> PLTEQEIDELCDEWVPEPLIPPITEDMKHEPPVLESAAGPHTTVNGKDVVNFASANYLGLIGHEKLLESCTSALEKYGVGSCGPRGFYGTIDVHLDCETRISKFLGTPDSILYSYGLSTMFSTIPCFCKKGDVIVADEGVHWGIQNGLQLSRSTIVYFKHNDMESLRITLEKIMTKYKRSKNLRRYIVAEAVYQNSGQIAPLDEIVKLKEKYRFRVILDESNSFGVLGRSGRGLAEHHSVPIEKIDVVTAAMGHALATEGGFCTGNARIIDYQRLSSSGYVFSASLPPYLASAAITAIDVIDQNPDMLVKLKQNVALLWKGLSDIKGMSLTSNRESPIVFLKLEKSSGSAKDDLLLLEKMADRALKEDSLLVVSSKRSFLDKCRLPVGIKLYVSAGHSESDLLKASESLKRLASELLLKS;> MYLTAVSTYFSYGLLFAFGQLRDFFRRFIDWWFTSNLQGYAPICLGHEDFYIRRLYHRIQDCFERPISSAPDAWFDVVERYSNDNNKTLKRTTKTSRCLNLGSYNYLGFGSFDEYCTPRVIESLKKFSASTCSSRVDAGTTSVHAELEECVTRFVGKPAAVVFGMGYATNSAIIPVLIGKGGLIISDSLNHSSIVNGARGSGATIRVFQHNTPSHLERVLREQIAEGQPRTHRPWKKIIVVVEGIYSMEGEICHLPEVVAICKKYKAYVYLDEAHSIGAIGKTGKGICELLGVDTADVDVMMGTFTKSFGSCGGYIAGSKELIQYLKHQCPAHLYATSIPTPSAQQIISAIKVILGEDGSNRGAQKLARIRENSNFFRAELQKMGFEVLGDNDSPVMPIMLYNPAKIPAFSRECLRQKVAVVVVGFPATPLLLARARICISASHSREDLIRALKVISKVGDLSGIKYFPAEPKKIEQSKNDIKLD;> MADYKDDDDKSGPDEVDASGRMNWVQRKIYLYNVTFGLYMLDWWERYLFNSLVVVLMWFVLYNGTRYFSELFQRHLT;> MANLYVKAVPPPDMNRNTEWFMYPGVWTTYMLILFFGWLVVLSVSGCSPGMAWTVVNLAHFVVTYHSFHWMKGTPFADDQGIYNGLTWWEQMDNGQQLTRNRKFLTLVPVVLYLIASHTTDYRHPWLFLNTLAVMVLVVAKFPNMHKVRIFGINGDK;> MASNLVEMFNAALNWVTMILESPSARVVLFGVPIRGHFFVEGLLGVVIIILLTRKSYKPPKR

The serine palmitoyltransferase (SPT) complex catalyzes the first and rate-limiting step in sphingolipid biosynthesis in all eukaryotes. ORM/ORMDL proteins are negative regulators of SPT that respond to cellular sphingolipid levels. We determined the cryo–electron microscopy structure of Arabidopsis SPT-ORM1 complex, composed of LCB1, LCB2a, SPTssa, and ORM1, in an inhibited state. The SPT-ORM1 complex is a ceramide sensor in the ER that controls cellular sphingolipid homeostasis.

The ORM1-dependent SPT repression is largely relieved by LCB2a-ΔN5 (deletion of residues 2 to 5) or ORM1-ΔN8 (deletion of residues 2 to 8). The LCB2a-ΔN5 and ORM1-ΔN8 variants were inhibited by C6-phytoceramide to a lesser degree than the WT AtSPT-ORM1 complex. These results suggest that the hybrid β sheet between ORM1 and LCB2a strengthens but is not absolutely required for the ORM1-dependent SPT inhibition. The flexible ORM1 N terminus is consistent with the greatly diminished ORM1-dependent SPT suppression for the LCB2a-ΔN5 variant. Together, these results suggest that both ceramide binding and the formation of a hybrid β sheet are critical for stabilizing the inhibitory conformation of the ORM1 N terminus.>MGSSHHHHHHSQDPSQFIRRDIAQTVNGSLTLTQQTNLSAPLVSSSTGEFGGSLAANRTFTIRNTGAPTSIVFEKGPASGANPAQSMSIRVWGNQFGGGSDTTRSTVFEVGDDTSHHFYSQRNKDGNIAFNINGTVMPININASGLMNVNGTATFGRSVTANGEFISKSANAFRAINGDYGFFIRNDASNTYFLLTAAGDQTGGFNGLRPLLINNQSGQITIGEGLIIAKGVTINSGGLTVNSRIRSQGTKTSDLYTRAPTSDTVGFWSIDINDSATYNQFPGYFKMVEKTNEVTGLPYLERGEEVKSPGTLTQFGNTLDSLYQDWITYPTTPEARTTRWTRTWQKTKNSWSSFVQVFDGGNPPQPSDIGALPSDNATMGNLTIRDFLRIGNVRIVPDPVNKTVKFEWVE[3x]

The proximal half-fiber is formed by a parallel homo-trimer of gp34. The protein is a highly intertwined trimer containing a 2 nm-wide triple β-helix domain interspersed with three wider domains in which each of the monomers forms an anti-parallel β-sheet. The long tail fibers recognize the outer membrane protein C (OmpC) or the lipopolysaccharide (LPS) of E. coli and are responsible for the initial and reversible attachment of the virion. The carboxy-terminal parts of gp34 that we crystallized occupy the part of the proximal tail fiber closest to gp35 (the “knee”).

Crystals belonging to two different space groups (P21 and R32) were obtained for gp34(894–1289). The obtained model was also refined against data collected to 2.0 Å resolution from a native crystal (i.e., not modified with selenomethionine) of the same crystal form (P21 space group), using the same test selection set for calculating the free R-factor selected in thin resolution shells. Here, the refined model contained the same protein residues as before, plus seven glycerol molecules and 1312 water molecules. Both the native and selenomethionine-modified models have good correspondence to the measured data and reasonable stereochemical parameters, although residues at the amino- and carboxy-termini have higher temperature factors and show some disorder.> MLTEGISIQSYDGHTFGALVGSPAKAPAPVIVIAHEILGVNAFMRETVSWLVDQGYAAVCPDLYARQAPGTALDPQDEAQREQAYKLWQAFDMEAGVGDLEAAIRYARHLPYSNGKVGLVGYSLGGALAFLVAAKGCVDRAVGYCGVGLEKQLDKVPEVKHPALFHMGGQDHFVPAPSRQLITEGFGANPLLQVHWYEG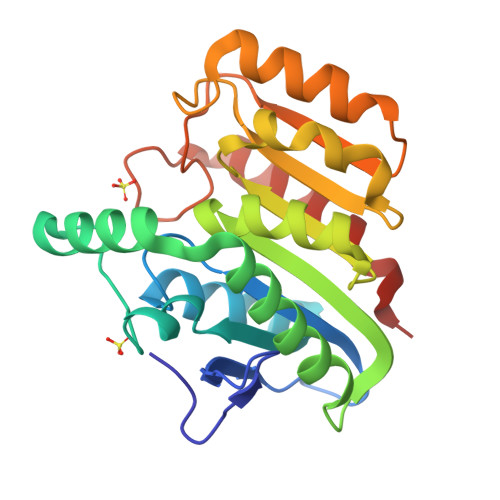AGHSFARTGSSDYVASAAALANERTLDFLAPLQSKKP>[2x]GPAGKATANAPTDAAITAASDFAALEKACAGR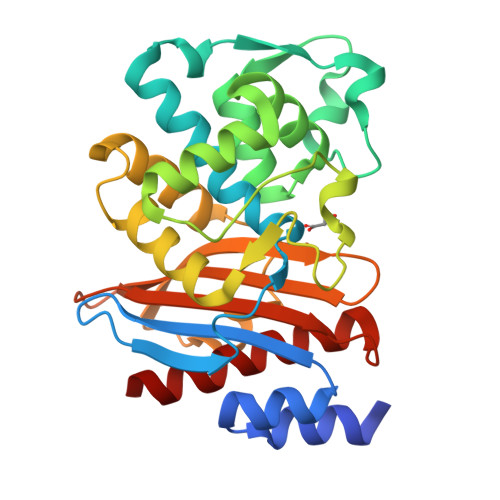LGVTLLDTASGRRIGHRQDERFPMCSTFKSMLAATVLSQAERMPALLDRRVPVGEADLLSHAPVTRRHAGKDMTVRDLCRATIITSDNTAANLLFGVVGGPPAVTAFLRASGDTVSRSDRLEPELNSFAKGDPRDTTTPAAMAATLQRVVLGEVLQPASRQQLADWLIDNETGDACLRAGLGKRWRVGDKTGSNGEDARNDIAVLWPVAGGAPWVLTAYLQAGAISYEQRASVLAQVGRIADRLIG>[2x]GMTSTSITAVEYQSKRLESRLLKETREYVIALPEGYAQSLEAYPVVYLLDGEDQFDHMASLLQFLSQGTMPQIPKVI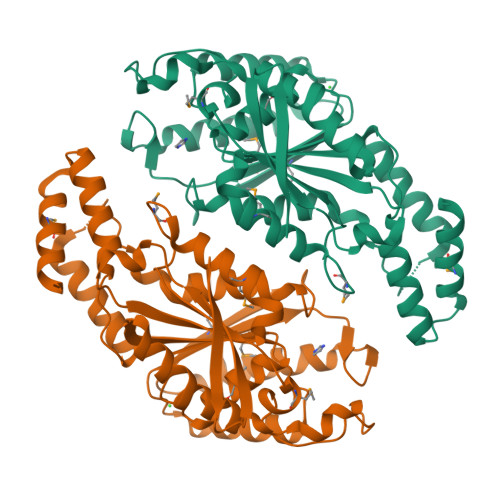IVGIHNTNRMRDYTPTHTLVLPSGNKGNPQYQHTGGAGRFLDFIEKELAPSIESQLRTNGINVLVGHSFGGLVAMEALRTDRPLFSAYLALDTSLWFDSPHYLTLLEERVVKGDFKQKQLFMAIANNPLSPGFGVSSYHKDLNLAFADKLTKLAPKGLGFMAKYYPEETHQSVSHIGLYDGIRHLFKDFAIDIYSDSFSKQQVIDQYGVLSERFGHKVTPSQQYLEQLIQYSDRQQLTERKQMLEGLRQHFAKD>[2x]GPYMIQEEEWDRD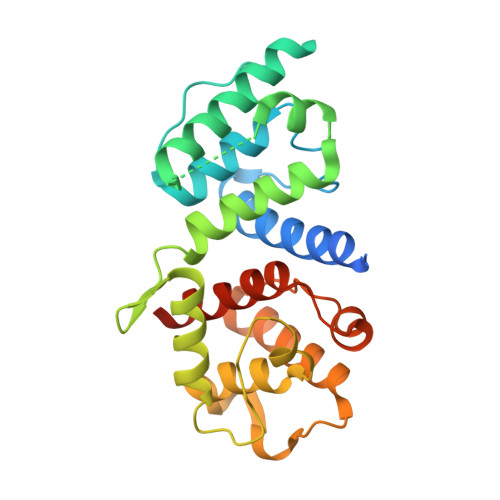LLLDPAWEKQQRKTFTAWCNSHLRKAGTQIENIEEDFRNGLKLMLLLEVISGERLPKPDRGKMRFHKIANVNKALDYIASKVVKLVSIGAEEIVDGNVKMTLGMIWTIILRFAIQDISVEETSAKEGLLLWCQRKTAPYRNVNIQNFHTSWKDGLGLCALIHRHRPDLIDYSKLNKDDPIGNINLAMEIAEKHLDIPKMLDAEDIVNTPKPDERAIMTYVSCFYHAFAGAEQAETAA> MQIQTPDWVKHAVFYQIFPDRFARSKQPRKRLLQEARWEDWDSMPTLQGYKGGDLWGIMEDLDYIQNLGINAIYFTPIFQSASNHRYHTHDYYQVDPMLGGNEAFKELLDAAHQRNIKVVLDGVFNHSSRGFFFFHDVLENGPHSPWVNWFKIEGWPLSPYNGEFPANYVGWAGNRALPEFNHDNPEVREYIMEIAEYWLKFGIDGWRLDVPFEIKTPGFWQEFRDRTKAINPEAYIVGEVWGDSRQWLDGTQFDGVMNYLFAGPTIAFAAGDRVVLEQVQSRDYQPYPPLFAAEYATKIQEVLQLYPWEIQLTQLNLLASHDTAR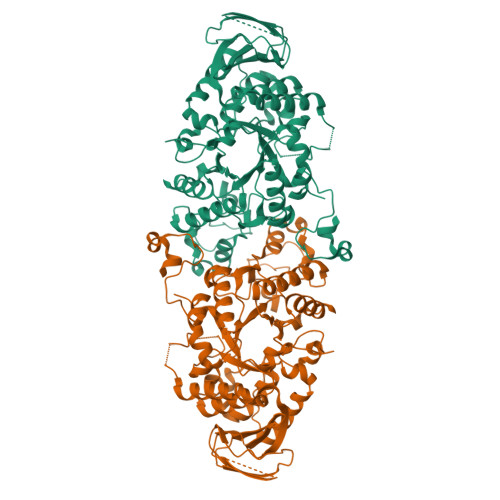LMTIAGGDIASVELSTLLLLTFPGAPSIYYGDEVGLPGGIDPDSRRGFPLEANWNQEIFNTHRQLITIRQTYPALRTGDYQVLYAQGQLYLFARTLGTEELIIAINAGTSSATANVDVASLHTQPNKLLYGTAEAEWNGEEGTQQLSLTLPARSGCILGTGD>[2x]MGNYKKPKLLYCSNGGHFLRILPDGTVDGTRDRSDQHIQLQLSAESVGEVYIKSTETGQYLAMDTDGLLYGSQTPNEECLFLERLEENHYNTYISKKHAEKNWFVGLKKNGSCKRGPRTHYGQKAILF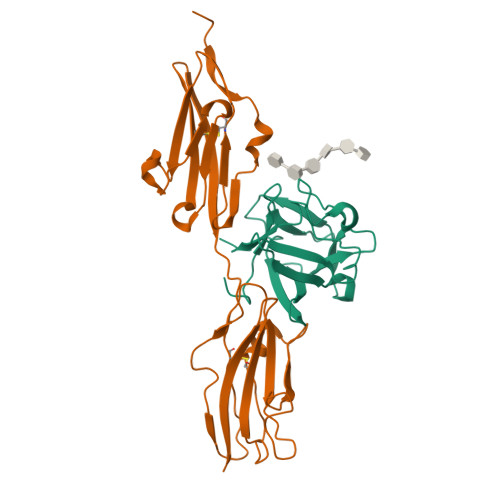LPLPVSSD;>MADNTKPNRMPVAPYWTSPEKMEKKLHAVPAAKTVKFKCPSSGTPQPTLRWLKNGKEFKPDHRIGGYKVRYATWSIIMDSVVPSDKGNYTCIVENEYGSINHTYQLDVVERSPHRPILQAGLPANKTVALGSNVEFMCKVYSDPQPHIQWLKHIEVNGSKIGPDNLPYVQILKTAGVNTTDKEMEVLHLRNVSFEDAGEYTCLAGNSIGLSHHSAWLTVLEALEER[2x]>MMSREADHTIKGFLYQFNKTLNSILSSTDQDEIQIEGIIEDIDIKNSNITNAIQCKYHESKVRHNLSDIYKPILQMLLHFLENDSLNIKYALYAYFPNEQVGVKEVTKSQIEEILSSSNFDYISKYISKIKPPKEQIIKELLGKTSKTTEDKTRIKKYYETSKLETIVDIDKFLRDHFVFEIGLSYEELMNETKNLLMKEGFSLEDVKDLFYPNSIQYIAELSILPEAEKRISSKNKLIDYLKGNKKTAMSRWTSEVLTRKQLLKVRKNQLVPSLNINSRSRYFIIDPDTIDNFDDEFILFVKDYLDKYNSKIKLHTETPCFILKTDVNNLSEYHKRFVSRNIQIITGYIGDTFYFKEFNKEPKRIIKDNWVEFKARISCNSDEVIKCINYKKCDDLYIVGGVDVSLLDTADVNIENLEINNFRELKYLLSMLKEI[12x];>[6x]MKIGSVIESSPHSILVKIDTLKIFEKAKSALQIGKYLKIQEGNHNFVLCVIQNIKISTDKDEDIFILTVQPVGIFKGEEFFQGNSMLPSPTEPVFLVEDDILNKIFSNEKTKIFHLGNLAQNEEVSFTLDGDKFFSKHVAVVGSTGSGKSCAVAKILQNVVGINDARNINKSDKKNSHIIIFDIHSEYKSAFEIDKNEDFNLNYLDVEKLKLPYWLMNSEELE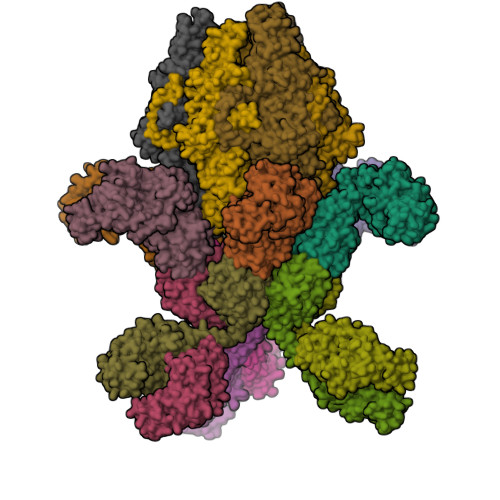TLFIESNEQNSHNQVSQFKRAVVLNKEKYNPEFKKITYDSPVYFNINEVFNYIYNLNEEVINKIEGEPSLPKLSNGELVENRQIYFNEKLEFTSSNTSKATKASNGPFNGEFNRFLSRFETKLTDKRLEFLLLNQDVEENSKYRTEHFEDILKQFMGYLDRSNVSIIDLSGIPFEVLSITISLISRLIFDFAFHYSKLQHQKDELNDIPFMIVCEEAHNYIPRTGGIEFKAAKKSIERIAKEGRKYGLSLMVVSQRPSEVSDTILSQCNNFINLRLTNINDQNYIKNLLPDNSRSISEILPTLGAGECLVVGDSTPIPSIVKLELPNPEPRSQSIKFHKKWSESWRTPSFEEVIMRWRKENG> 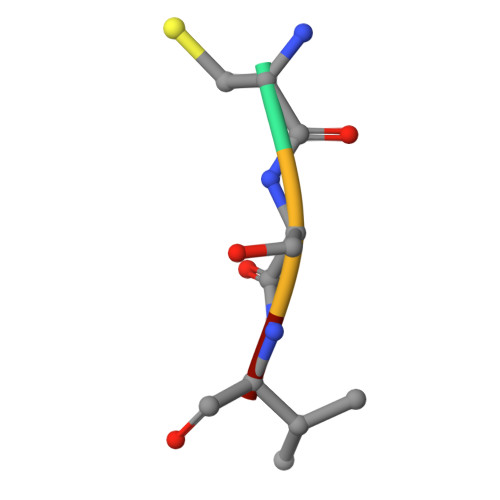CSIM> ENPYERGPDPTESSIEAVRGPFAVAQTTVSRLQADGFGGGTIYYPTDTSQGTFGAV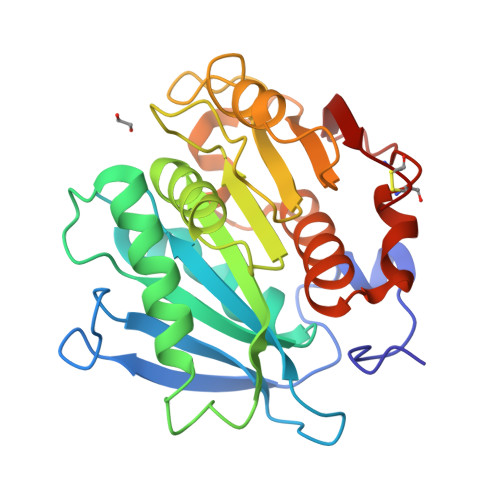AISPGFTAGQESIAWLGPRIASQGFVVITIDTITRLDQPDSRGRQLQAALDHLRTNSVVRNRIDPNRMAVMGHSMGGGGALSAAANNTSLEAAIPLQGWHTRKNWSSVRTPTLVVGAQLDTIAPVSSHSEAFYNSLPSDLDKAYMELRGASHFVSNTPDTTTAKYSIAWLKRFVDNDLRYEQFLCPAPDDFAISEYRATCPF1,5-anhydro-2,3,4-trideoxy-3-{[(4S)-3,3-dimethyl-1-(8-methylquinolin-2-yl)piperidine-4-carbonyl]amino}-D-erythro-hexitol 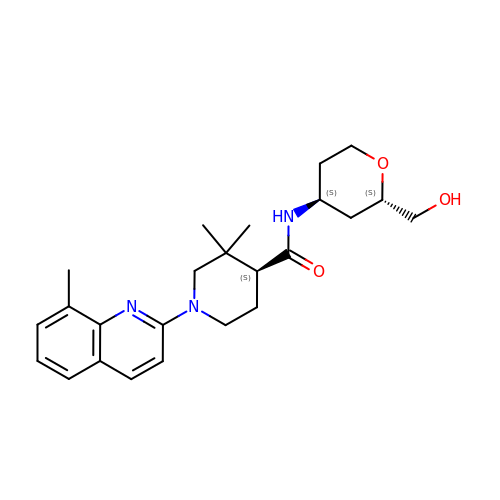| C24 H33 N3 O3 | OLJFTJILJDDJGV-SLFFLAALSA-N>[4x]DPAVTYY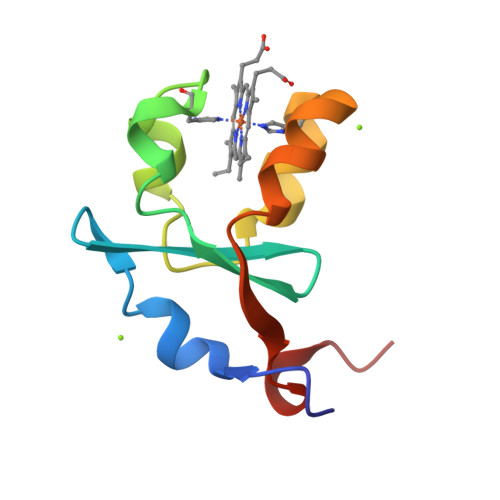RLEEVAKRNTSEETWMVIHGRVYDLTRFLSEHPGGEEVLREQAGADATESFEDVGHSPDAREMLKQYYIGDVHPNDLKPK Under osmotic stress, bacteria express a heterotetrameric protein complex, KdpFABC, which functions as an ATP-dependent K+ pump to maintain intracellular potassium levels. The subunit KdpA belongs to the Superfamily of K+ Transporters and adopts a pseudo-tetrameric architecture with a membrane embedded selectivity filter as seen in K+ channels. KdpB belongs to the superfamily of P-type ATPases with a conserved binding site for ions within the membrane domain and three cytoplasmic domains that orchestrate ATP hydrolysis via an aspartyl phosphate intermediate. Previous work has hypothesized that K+ moves parallel to the membrane plane through a 40-Å long tunnel that connects the selectivity filter of KdpA with a canonical binding site in KdpB.

In addition, the structure was obtained under the most native conditions to date, namely with uninhibited, wild-type (WT) protein embedded in lipid bilayer nanodiscs under active turnover conditions induced by the addition of K+ and ATP. We also determined a cryo-EM structure at substantially higher resolution (2.1 Å) compared to previous structural studies. Map densities in the catalytic domains of KdpB unambigiously show phosphorylation of Asp307 in the P-domain and binding of ADP together with two Mg2+ ions in the nucleotide binding domain (N-domain), confirming the conformation to be E1~P·ADP. Unlike previous structures, our map resolves most of the N-terminus of KdpB, revealing a potential interaction involving Glu161 from the A-domain, Arg3 from the N-terminus as well as Asp552 and Lys557 from the P-domain. In the current map, however, clear densities are visible at all four sites, likely due to increased resolution, but density at S3 remains much stronger. There are many side chain oxygen atoms in this region that produce a generally hydrophilic environment and our new structure reveals numerous discrete densities within this cavity. Because their magnitude is comparable to or lower than the surrounding protein side chains we model them as water molecules, thus producing a highly hydrated vestibule. Whereas previous structures show 5–7 discrete densities extending from the vestibule into the tunnel, our new structure reveals ~17 spherical densities in this region, all of comparable strength to the surrounding protein density. These densities, which we have modeled as water, are most prevalent near the vestibule, which is the wider part of the tunnel, but then disappear completely at the subunit interface near Phe232, which is the narrowest part of the tunnel and also distinctly hydrophobic. Our higher resolution map shows an exceedingly strong, wellresolved density at the canonical binding site along the axis of the unwound M4 helix, providing compelling evidence that, like other P-type pumps, the transport ion is bound at this canonical site in this state.

> MAAQGFLLIATFLLVLMVLARPLGSGLARLINDIPLPGTTGVERVLFRALGVSDREMNWKQYLCAILGLNMLGLAVLFFMLLGQHYLPLNPQQLPGLSWDLALNTAVSFVTNTNWQSYSGETTLSYFSQMAGLTVQNFLSAASGIAVIFALIRAFTRQSMSTLGNAWVDLLRITLWVLVPVALLIALFFIQQGALQNFLPYQAVNTVEGAQQLLPMGPVASQEAIKMLGTNGGGFFNANSSHPFENPTALTNFVQMLAIFLIPTALCFAFGEVMGDRRQGRMLLWAMSVIFVICVGVVMWAEVQGNPHLLALGTDSSINMEGKESRFGVLVSSLFAVVTTAASCGAVIAMHDSFTALGGMVPMWLMQIGEVVFGGVGSGLYGMMLFVLLAVFIAGLMIGRTPEYLGKKIDVREMKLTALAILVTPTLVLMGAALAMMTDAGRSAMLNPGPHGFSEVLYAVSSAANNNGSAFAGLSANSPFWNCLLAFCMFVGRFGVIIPVMAIAGSLVSKKSQAASSGTLPTHGPLFVGLLIGTVLLVGALTFIPALALGPVAEYLS;> MSRKQLALFEPTLVVQALKEAVKKLNPQAQWRNPVMFIVWIGSLLTTCISIAMASGAMPGNALFSAAISGWLWITVLFANFAEALAEGRSKAQANSLKGVKKTAFARKLREPKYGAAADKVPADQLRKGDIVLVEAGDIIPCDGEVIEGGASVDESAITGESAPVIRESGGDFASVTGGTRILSDWLVIECSVNPGETFLDRMIAMVEGAQRRKTPNEIALTILLIALTIVFLLATATLWPFSAWGGNAVSVTVLVALLVCLIPTTIGGLLSAIGVAGMSRMLGANVIATSGRAVEAAGDVDVLLLDKTGTITLGNRQASEFIPAQGVDEKTLADAAQLASLADETPEGRSIVILAKQRFNLRERDVQSLHATFVPFTAQSRMSGINIDNRMIRKGSVDAIRRHVEANGGHFPTDVDQKVDQVARQGATPLVVVEGSRVLGVIALKDIVKGGIKERFAQLRKMGIKTVMITGDNRLTAAAIAAEAGVDDFLAEATPEAKLALIRQYQAEGRLVAMTGDGTNDAPALAQADVAVAMNSGTQAAKEAGNMVDLDSNPTKLIEVVHIGKQMLMTRGSLTTFSIANDVAKYFAIIPAAFAATYPQLNALNIMCLHSPDSAILSAVIFNALIIVFLIPLALKGVSYKPLTASAMLRRNLWIYGLGGLLVPFIGIKVIDLLLTVCGLV;> MSGLRPALSTFIFLLLITGGVYPLLTTVLGQWWFPWQANGSLIREGDTVRGSALIGQNFTGNGYFHGRPSATAEMPYNPQASGGSNLAVSNPELDKLIAARVAALRAANPDASASVPVELVTASASGLDNNITPQAAAWQIPRVAKARNLSVEQLTQLIAKYSQQPLVKYIGQPVVNIVELNLALDKLDEGTGLVPRGSSHHHHHHHH;> MSAGVITGVLLVFLLLGYLVYALINAEAF> SNELPSLCMLNNSFYYMRGGVNTFLIRVSDISVLMKEYDVSIYEPEDLGNCLNKSDS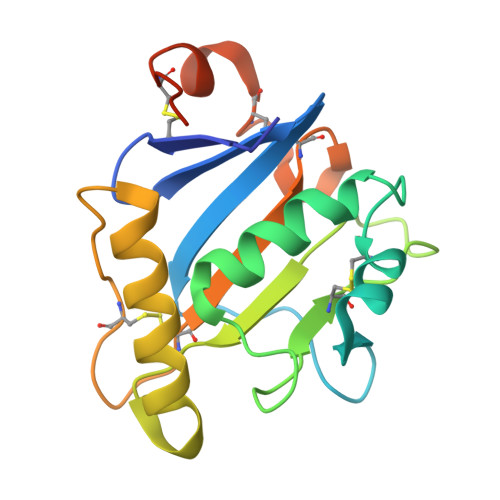SWAIHWFSNALGHDWLMDPPMLCRNKTKKEGSNIQFNISKADDARVYGKKIRNGMRHLFRGFHDPCEEGKVCYLTINQCGDPSSFDYCGVNHLSKCQFDHVNTGSHHHHHH>MGHHHHHHGSTTQRNAQIAMGRKKFNMDPKKGIQFLIENDLLQSSPEDVAQFLYKGEGLNKTVIGDYLGERDDFNIKVLQAFVELHEFADLNLVQALRQFLWSFRLPGEAQKIDRMMEAFASRYCLCNPGVFQSTDTCYVLSFAIIMLNTSLHNHNVRDKPTAERFITMNRGINEGGDLPEELLRNLYESIKNEPFKIPEDDGNDLTHTFFNPDREGWLLKLGGRVKTWKRRWFILTDNCLYYFEYTTDKEPRGIIPLENLSIREVEDPRKPNCFELYNPSHKGQVIKACKTEADGRVVEGNHVVYRISAPSPEEKEEWMKSIKASISRDPFYDMLATRK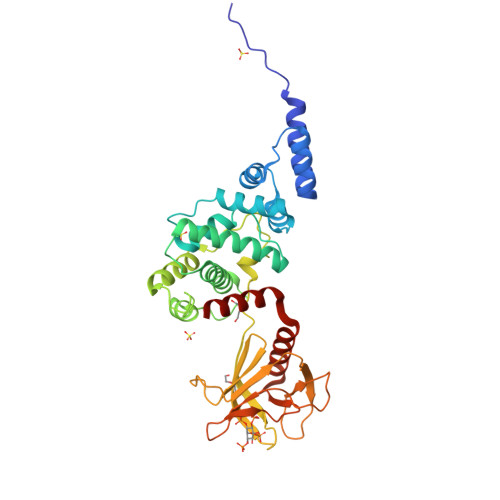RRIANKK[2x]>SGISLDNSYKMDYPEMGLCIIINNKNFHKSTGMTSRSGTDVDAANLRETFRNLKYEVRNKNDLTREEIVELMRDVSKEDHSKRSSFVCVLLSHGEEGIIFGTNGPVDLKKITNFFRGDRCRSLTGKPKLFIIQACRGTELDCGIET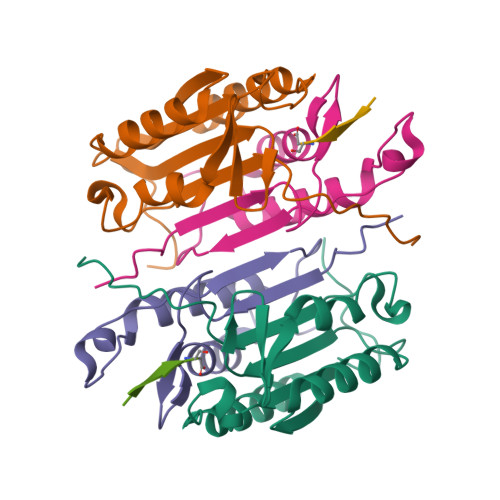D[2x];>[2x]SGVDDDMACHKIPVEADFLYAYSTAPGYYSWRNSKDGSWFIQSLCAMLKQYADKLEFMHILTRVNRKVATEFESFSFDATFHAKKQIPCIVSMLTKELYFYHHHHHHH;>[2x]XLDESD>ASQTITVGSWGGPG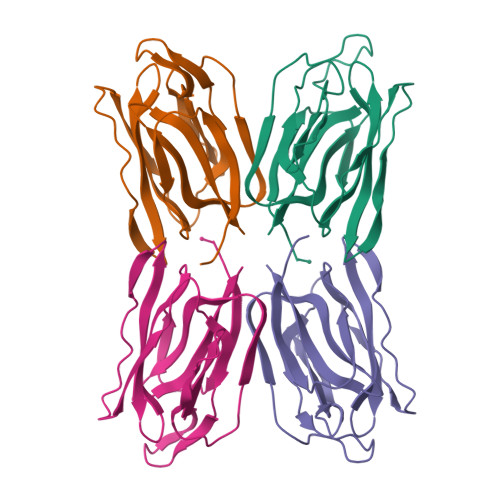GNGWDEGSYTGIRQIELSYKEAIGSFSVIYDLNGDPFSGPKHTSKLPYKNVKIELKFPDEFLESVSGYTGPFSALATPTPVVRSLTFKTNKGRTFGPYGDEEGTYFNLPIENGLIVGFKGRTGDLLDAIGIHMSL[4x]OphP is an essential enzyme for the biosynthesis of the macrocyclic peptide natural product omphalotin A. The enzyme has been proposed to proteolytically release a peptide intermediate from the precursor protein OphMA and to macrocyclize the multiply α-N-methylated core of this intermediate to produce omphalotin A. Our *in vitro* experiments demonstrate that OphP does not process OphMA but shows robust macrocyclase activity on pre-processed α-N-methylated peptides. OphP tolerates sequence promiscuity in the substrate but has a preference for highly α-N-methylated substrates and for N-methylated glycine residue at the catalytic site. The promiscuity of OphP is explained by structural analysis of co-complexes which reveals a predominantly hydrophobic substrate binding cleft with few interactions between substrate side chains and OphP. Similar to other POPs, the monomer has two domains, an α/β hydrolase domain (residues 1–82, 453–738) and the seven-bladed β-propeller domain (residues 83–452) ([Fig fig4]).

We determined the covalent complex structure of OphP with ZPP by soaking wild-type OphP crystals with 5 mM ZPP overnight. The structure of the complex was determined at 2.0 Å resolution. Additional electron density, which we fitted as ZPP covalently linked to S580 (**Figure S11**) was seen in two subunits. The other two subunits had weak electron density suggesting low occupancy. The overall structure of the OphP:ZPP complex is largely unchanged from the apo structure of S580A (0.5 Å over 716 Cα atoms) (**Figure 4-Figure supplement 2**). There are differences in loops Leu139–Ala146, Ser164–Met171, Ser179– Met195, Pro222–Gly230, Leu696–Ser706 and Ala622–Tyr664. As a result, His701 has moved closer (7.6 Å to serine) to both Asp665 and Ser580 to form the catalytic triad (**Figure 4-Figure supplement 2**). The carbonyl at P1 proline of the ZPP(acyl)-enzyme intermediate hydrogen bonds to the backbone amide of Asn581 and the side chain hydroxyl of Tyr499. The benzene ring of ZPP is located in an aromatic hydrophobic pocket. These results confirm Ser580 as the key catalytic residue and suggest a structural re-arrangement of active site residues including His701 upon substrate binding. The OphP:ZPP complex has a proline group at the P1 site which results in Ile606 adopting an unfavorable conformation ([Fig fig5]). The requirement for the structural re-arrangement of Ile606 correlates with the lower-than-expected potency of ZPP as an inhibitor against OphP.

>[4x]MSFPGWGPYPPVERDETSAITYSSKLHGSVTVRDPYSQLEVPFEDSEETKAFVHSQRKFARTYLDENPDREAWLETLKKSWNYRRFSALKPESDGHYYFEYNDGLQSQLSLYRVRMGEEDTVLTESGPGGELFFNPNLLSLDGNAALTGFVMSPCGNYWAYGVSEHGSDWMSIYVRKTSSPHLPSQERGKDPGRMNDKIRHVRFFIVSWTSDSKGFFYSRYPPEDDEGKGNAPAMNCMVYYHRIGEDQESDVLVHEDPEHPFWISSVQLTPSGRYILFAASRDASHTQLVKIADLHENDIGTNMKWKNLHDPWEARFTIVGDEGSKIYFMTNLKAKNYKVATFDANHPDEGLTTLIAEDPNAFLVSASIHAQDKLLLVYLRNASHEIHIRDLTTGKPLGRIFEDLLGQFMVSGRRQDNDIFVLFSSFLSPGTVYRYTFGEEKGYRSLFRAISIPGLNLDDFMTESVFYPSKDGTSVHMFITRPKDVLLDGTSPVLQYGYGGFSLAMLPTFSLSTLLFCKIYRAIYAIPNIRGGSEYGESWHREGMLDKKQNVFDDFNAATEWLIANKYASKDRIAIRGGSNGGVLTTACANQAPGLYRCVITIEGIIDMLRFPKFTFGASWRSEYGDPEDPEDFDFIFKYSPYHNIPPPGDTVMPAMLFFTAAYDDRVSPLHTFKHVAALQHNFPKGPNPCLMRIDLNSGHFAGKSTQEMLEETADEYSFIGKSMGLTMQTQGSVDSSRWSCVTV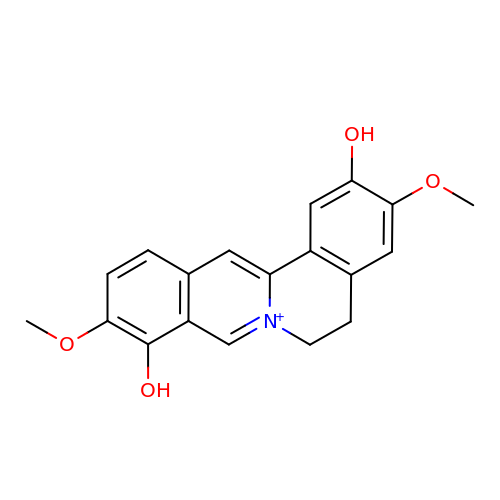2,9-dihydroxy-3,10-dimethoxy-5,6-dihydroisoquino[3,2-a]isoquinolinium | C19 H18 N O4 | DRAPVRZDBZHUPL-UHFFFAOYSA-O>[2x]KEWQENKSWNAHFTEHKSQGVVVLWNENKQ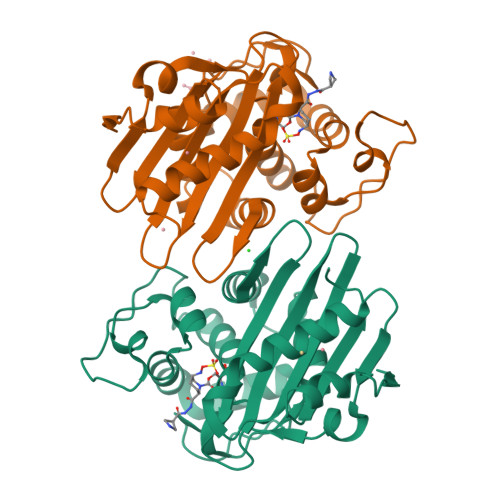QGFTNNLKRANQAFLPASTFKIPNSLIALDLGVVKDEHQVFKWDGQTRDIATWNRDHNLITAMKYSVVPVYQEFARQIGEARMSKMLHAFDYGNEDISGNVDSFWLDGGIRISATEQISFLRKLYHNKLHVSERSQRIVKQAMLTEANGDYIIRAKTGYSTRIEPKIGWWVGWVELDDNVWFFAMNMDMPTSDGLGLRQAITKEVLKQEKIIP> MINDMHPSL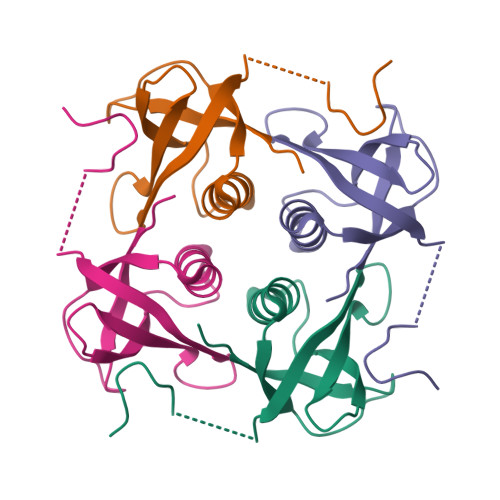IKDKDIVDDVMLRSCKIIAMKVMPDKVMQVMVTVLMHDGVCEEMLLKWNLLDNRGMAIYKVLMEALCAKKDVKISTVGKVGPLGCDYINCVEISM> MDDSSDEDNLLFDDLQSLHVATPLLHAPNLTKELECNVFLKMENIQPSGSVKMRGIGAFCYQAVQTRGTNIQFVCGSGPNTVLAVSYCARQLGVEAIIV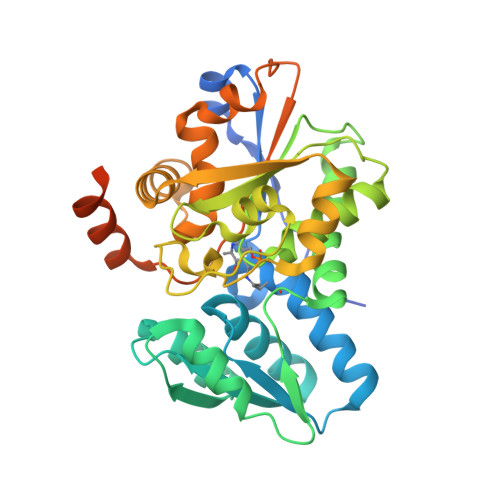VPKATNERICQSIRTDGSHLILYGENWTAAEVHARKLVRRNGIYVPSSDHALIWQGHSTIVQELKTQLNDNPPAAIICPVGGGGLLNGVIMGLQEADWKDVPVIAVETHGSNAFQASVVAGELVIMEKNNTIATSLISKAVSSKSLELSLNHPVVPFAVSDAMAADAVRLFAEDFKMLVEASAGAALSLCYTHLIRDILPSLSPAKDVVVLVTGGSDISLAHLDEYRKKYMHPAVVVKSGSEIFMKMDNTLQSVADVDPENVDVHSS> MSTLNKHISIPKDMSSKDDLDFHFLREEGIRYIKELGSNFWTDYNTHDPGITMLEVLCYAISDLGNRINIPIEDLIANEEGGVKGQFYKVQEILPSAPTSELDLRKLFIDIEGIKNCWIKRERVTVFADLKNQKLSYEKTIWEDLKENQKAQFDLKGLYRILVETEDADKVLSESLEKAVFTKFHANRNLCEDLIKVEKVATEPISVCANVEVAPEADEELIHAQILIAIEDYLAPSPRHYSLKQMVDKGYTMDEIFEGPFLENGFIDTVELKASELRKEVRLSDIINIIMSIDGVKIVKEITLGNCDENDGIENNQWVICIPENKKPKLCKKTTINYFKGILPINLNPVRVDNHKSKILASRLENDLKAKDDLEPAIPQGTFADWGEYSSIQHEFPETYGISDIGLPPKLGVKRAVLARQLKGYLLFFDQILASYFEHLSKIKSLLSLDQGPSFTYFTQAIKDIKDVEELFKDPTLLENDEELTKSLIGKLDDTIERRNQLMDHLIARFAENFSSYAFLMKFLYGESTDEIVLQDKQSFLREYKEISRERGEGFNFYEQSNDNLWDTLNVSGAQKRISKLVGVKDYSRRNLSDTAVEIYRYEHVDGNWVYRWRIRDENGKVLLSATTSYPTYNSAGNEMYFAILKILETPLSDLEKLLEVNFRNENEAGSFHFHKAATSNKFSFDIINPVIDSESSSDFIVAKQYTYYPDRTQAVLGAISLLNFIKYTFTEEGIYLVEHILLRPSPLDPEYLAMQTDAGKEYIEGNFLPFCSDDYENCKMIDPYSFRVSIVLPGFTYRFANKDFRDYLENLIREELPAHIVAKICWIGYRKGEEPELFQEDVENP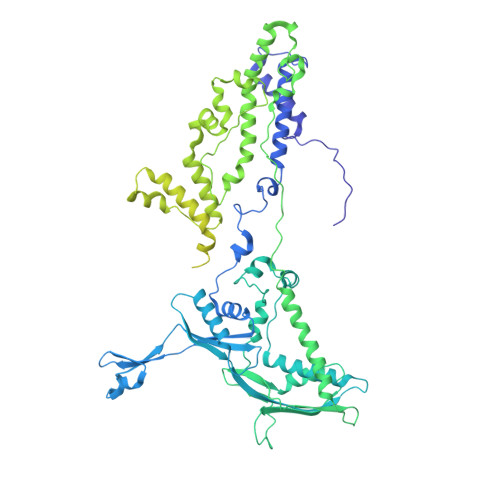ETPIFKENQLEIFEKAYKNYLFELTDIHKRKGFIASMNKYNQVLNEMTSSLTGLHTIYPTGRLYDCEDEEEELDGKLILGKTNLGTL> MHHHHH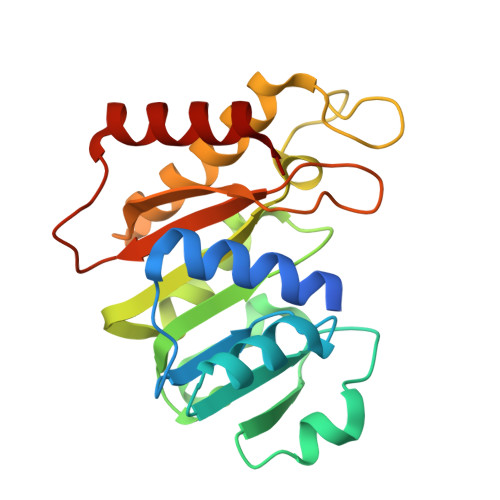HASGLVPRGSRGAHKLVGALEAFAIAVAGRRCLDAGASTGGFTEVLLDRGAAHVVAADVGYGQLAWSLRNDPRVVVLERTNARGLTPEAIGGRVDLVVADLSFISLATVLPALVGCASRDADIVPLVKPQFEVGKGQVGPGGVVHDPQLRARSVLAVARRAQELGWHSVGVKASPLPGPSGNVEYFLWLRTQTDRALSAKGLEDAVHRAISEGP>GSHMSTINYDLSRIKALAFDVDGVLSSTTVPLHPSGEPMRTVNIKDGYAIQLAVKKGLHIAIITGGRTEAVRIRFAALGVKDLYMGSAVKIHDYRNFRDKYGLSDDEILYMGDDVPDIEVMRECGLPCCPKDAVPEVKSVAKYISYADGGRGCGRDVVEQVLKAHGKWM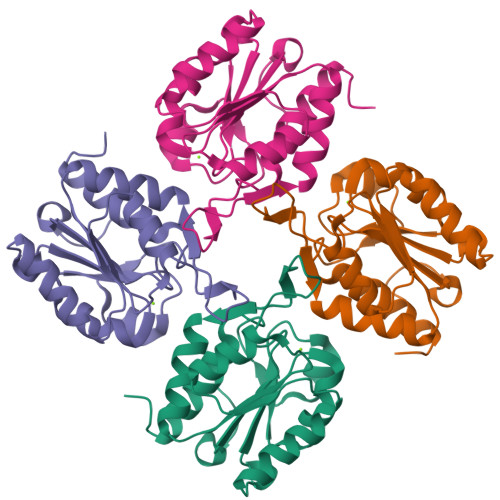AEDAFGW[4x]>MNDYSRQNFQDLNLFRGLGEDPAYHPPVLTDRPRDWPLDRWAEAPRDLGYSDFSPYQWRGLRMLKDPDTQAVYHDMLWELRPRTIVELGVYNGGSLAWFRDLTKIMGIDCQVIGIDRDLSRCQIPASDMENITLHQGDCSDLTTFEHLREMAHPLIFIDNAHANTFNIMKWAVDHLLEEGDYFIIEDMIPYWYRYAPQLFSEYLGAFRDVLSMDMLYANASSQLDRGVLRRVA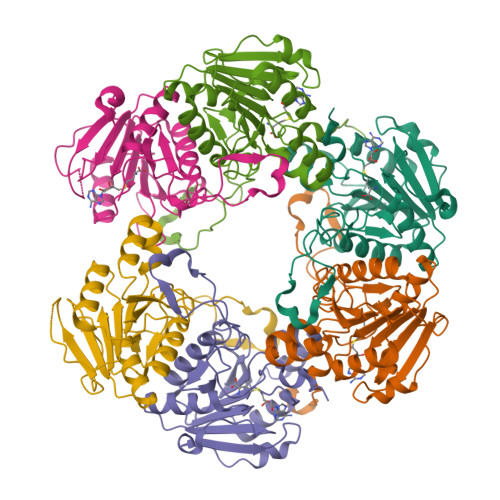AKQ[6x]>[8x]MRGSHHHHHHGSMSVSEIFVELQGFLAAEQDIREEIRKVVQSLEQTAREILTLLQGVHQGAGFQDIPKRCLKAREHFGTVKTHLTSLKTKFPAEQYYRFHEHWRFVLQRLVFLA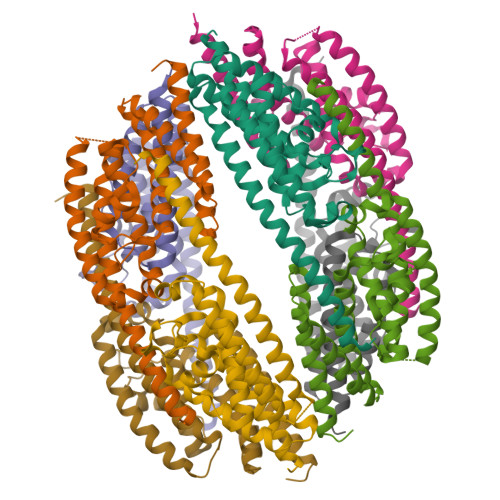AFVVYLETETLVTREAVTEILGIEPDREKGFHLDVEDYLSGVLILASELSRLSVNSVTAGDYSRPLHISTFINELDSGFRLLNLKNDSLRKRYDGLKYDVKKVEEVVYDLSIRGFNKETAAACVEK>[2x]MGEIRPTIGQQMETGDQRFGDLVFRQLAPNVWQHTSYLDM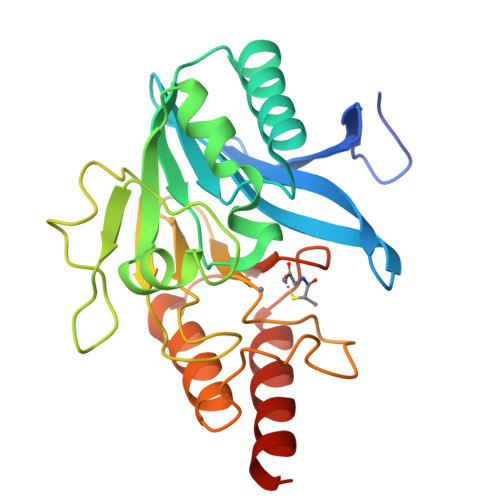PGFGAVASNGLIVRDGGRVLVVDTAWTDDQTAQILNWIKQEINLPVALAVVTHAHQDKMGGMDALHAAGIATYANALSNQLAPQEGMVAAQHSLTFAANGWVEPATAPNFGPLKVFYPGPGHTSDNITVGIDGTDIAFGGCLIKDSKAKSLGNLGDADTEHYAASARAFGAAFPKASMIVMSHSAPDSRAAITHTARMADKLRLEHHHHHH>[11x]AATTVNG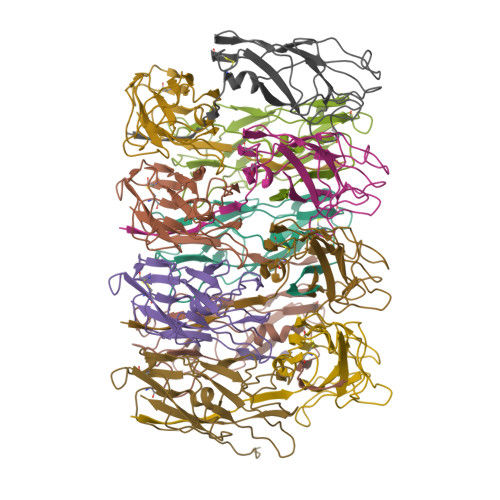GTVHFKGEVVNAACAVDAGSVDQTVQLGQVRTASLAQEGATSSAVGFNIQLNDCDTNVASKAAVAFLGTAIDAGHTNVLALQSSAAGSATNVGVQILDRTGAALTLDGATFSSETTLNNGTNTIPFQARYFATGAATPGAANADATFKVQYQ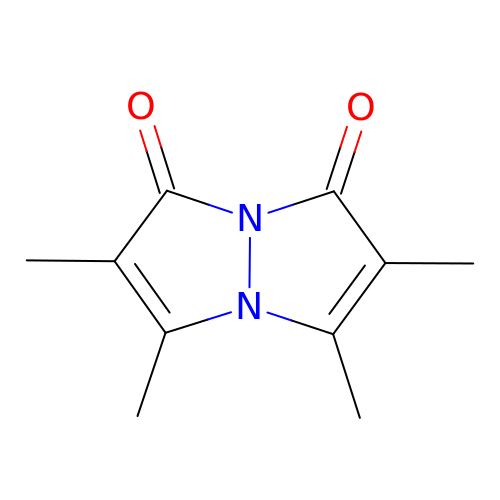2,3,5,6-tetramethyl-1H,7H-pyrazolo[1,2-a]pyrazole-1,7-dione | C10 H12 N2 O2 | VWKNUUOGGLNRNZ-UHFFFAOYSA-N> GSHGGSEFMISVADLDYASRKSSIFLFAPHVGTFTKQSMDKLVRPLAASAHRDWILDTVAGLPTYWDALAVKIPNIGNAIPGRRQLTDLDTWFRHGAGDVTQDDATLPSIVVGPLVVLIQLTQYWRYLELTRPDHLEDSADLQADVVTRQTQPGAKVETLGFCAGLLAAVAVASAGNRQEFQKYGAVAVRLAMMAGALIDGQEARDKATRDGGSVSYAIAWRGQKPGEEAARIVKDLNPNAYFAVLYDEA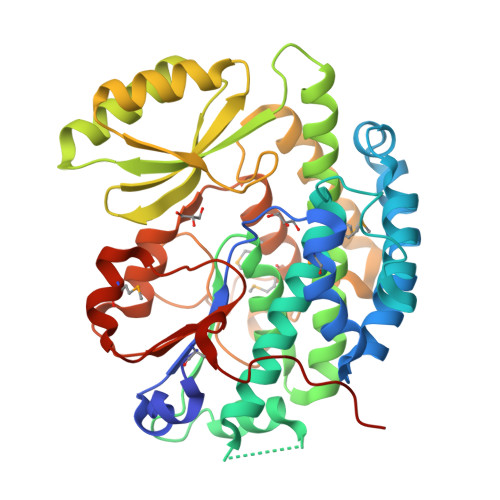RATVTTTRRTAPSLVNRLRAADVTVAEIGIKGRIHSPDSERKNNTDLLVDLCKSFEDLQYADAASLALPTYNNEAEGRPVSRDRGNMTEMVIRAILVNQCNWYGTFKGATEGREPFVVTLGLERSVPPTLMRSLGPHQVHYEDLADNGIPPAPQSP>[2x]MSLDSRLPAFRNLSPAARLDHIGQLLGLSHDDVSLLANAGALPMDIANGMIENVIGTFELPYAVASNFQINGRDVLVPLVVEEPSIVAAASYMAKLARANGGFTTSSSAPLMHAQVQIVGIQDPLNARLSLLRRKDEIIELANRKDQLLNSLGGGCRDIEVHTFADTPRGPMLVA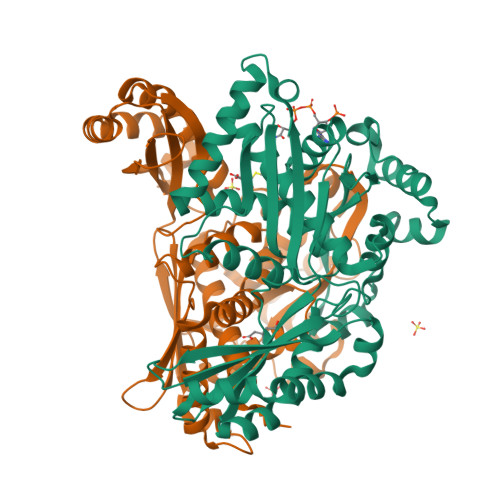HLIVDVRDAMGANTVNTMAEAVAPLMEAITGGQVRLRILSNLADLRLARAQVRITPQQLETAEFSGEAVIEGILDAYAFAAVDPYRAATHNKGIMNGIDPLIVATGNDWRAVEAGAHAYACRSGHYGSLTTWEKDNNGHLVGTLEMPMPVGLVGGATKTHPLAQLSLRILGVKTAQALAEIAVAVGLAQNLGAMRALATEGIQRGHMALHARNIAVVAGARGDEVDWVARQLVEYHDVRADRAVALLKQKRGQ The adaptor protein paxillin contains five conserved leucine-rich (LD) motifs that interact with a variety of focal adhesion proteins, such as α-parvin. α-parvin (Olski et al., 2001), also known as actopaxin or CH-ILKBP (Tu et al., 2001), is part of the ILK signaling complex (Tu et al., 2001), plays an essential role in adhesion-dependent PKB/Act activation (Fukuda et al., 2003) and in the regulation of actin organization (LaLonde et al., 2005) and Rac activation (LaLonde et al., 2005; Zhang et al., 2004). It belongs to the highly conserved parvin family that shares a common architecture composed of a variable N-terminal region followed by two CH domains (Olski et al., 2001). Our results demonstrate that full-length α-parvin contains a single LD binding site, formed by the N-linker helix, helix A, and helix G of the C-terminal type-5 CH domain.

To elucidate the molecular basis for LD recognition by α-parvin-CHC, we cocrystallized α-parvin-CHC with peptides representing the high-affinity ligands LD1, LD2, and LD4. The refined structures include residues 247–372 of α-parvin and paxillin residues 1–14, 141–155, and 262–274 for LD1, LD2, and LD4, respectively. All three LD motifs bind to the same binding site on α-parvin-CHC formed by the N-linker helix, the N-terminal part of helix A and the C-terminal part of helix G, which is consistent with our results from chemical shift mapping. Surprisingly, however, the orientation of LD1 is reversed compared to LD2 and LD4 in the corresponding crystal structures. Despite their antiparallel orientations, however, the binding modes of different LD peptides are very similar. The side chains of their conserved leucine residues in position 0, +3, +4, and +7 interact with a hydrophobic patch on the surface of the CHC domain formed by residues from the N-linker helix (A249, F250, L253, A257), helix A (V263, V264, and L268) and helix G (Y362 and F365). In addition, two positively charged residues (K260 and R369) of α-parvin-CHC are in close proximity to negatively charged residues of the bound LD peptides. Note that these electrostatic contacts involve the conserved aspartate D+1 of the LD consensus in the case of LD2 and LD4, whereas D+6 and E+8 are utilized in LD1. Consistent with their similar binding modes, all three LD peptides, irrespective of directionality, impose similar conformational changes in the N-terminal region of α-parvin-CHC, whereas the protein core remains virtually unperturbed. Residues 258–260 of helix A, which are α-helical in the unbound conformation, adopt a 310-helix in the complexes.

> NLSELDRLLLELNAVQHNPP;> SGRHERDAFDTLFDHAPDKLNVVKKTLITFVNKHLNKLNLEVTELETQFADGVYLVLLMGLLEGYFVPLHSFFLTPDSFEQKVLNVSFAFELMQDGGLEKPKPRPEDIVNCDLKSTLRVLYNLFTKYRNVE2'-deoxy-5'-O-[(R)-{[(R)-{[(1S,3R,4R,5S)-3,4-dihydroxy-5-methylcyclohexyl]oxy}(hydroxy)phosphoryl]oxy}(hydroxy)phosphoryl]-3,4-dihydrothymidine 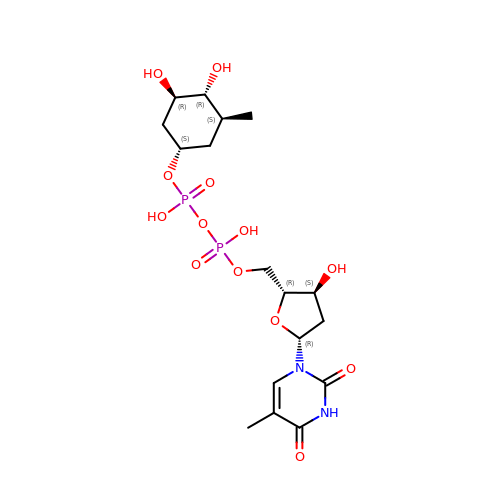| C17 H28 N2 O13 P2 | CWVOKCJHBPKJQP-PVMIAKCWSA-N> GHMWQENKSWNAHFTEHKSQGVVVLWNENKQQGFTNNLKRANQA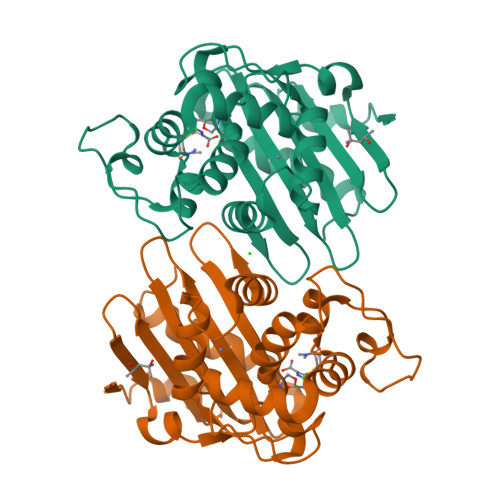FLPASTFAIPNSLIALDLGVVKDEHQVFKWDGQTRDIATWNRDHNLITAMKYSVVPVYQEFARQIGEARMSKMLHAFDYGNEDISGNVDSFWLDGGIRISATEQISFLRKLYHNKLHVSERSQRIVKQAMLTEANGDYIIRAKTGYDTKIGWWVGWVELDDNVWFFAMNMDMPTSDGLGLRQAITKEVLKQEKIIP methyl 5-(4-oxidanylidene-5~{H}-furo[3,2-c]pyridin-2-yl)pyridine-3-carboxylate 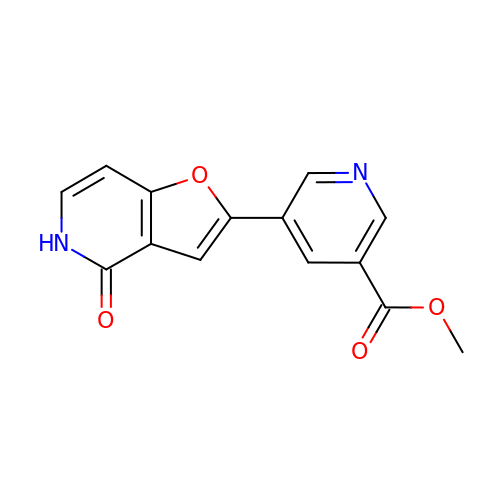| C14 H10 N2 O4 | CKTWBGKZILYBCF-UHFFFAOYSA-N> FLGKIWPSH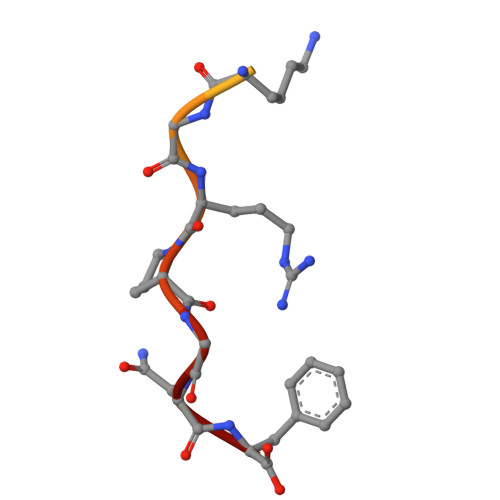KGRPGNF> XGLCALRSELQALRREGFSPEELAALESELQALERELA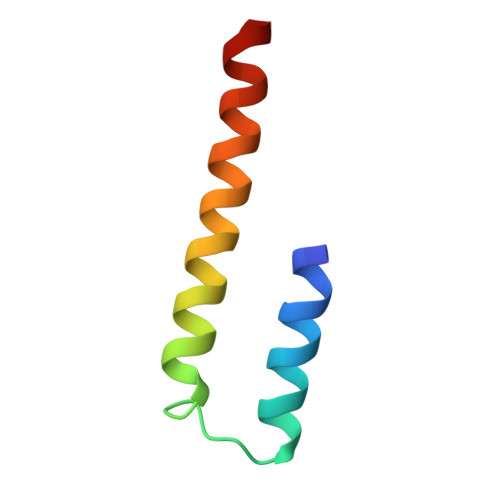ALRSELQALRGX3beta-(2-Diethylaminoethoxy)androst-5-en-17-one | C25 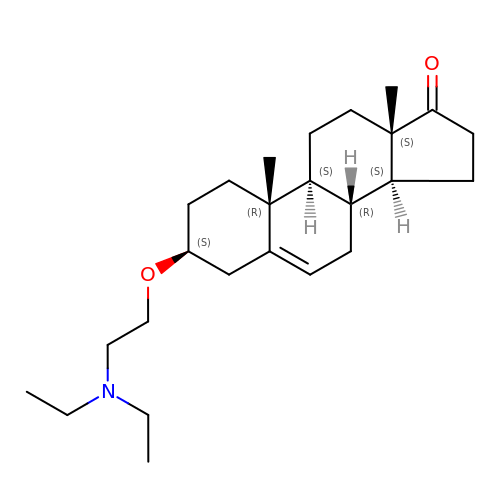H41 N O2 | DMZCCFMMPHJWQY-BKWLFHPQSA-N> MAHHHHHHSAAISNLQEKQTDFGMRVFSQVAQNSKGSNLAFSPYGVATILAMAQLGAGGNTLKTLNAKLGFSLQERGMARQQRLLQRDISSEEGVELASGVMVERKMALEKGFRRGLGKAFQASPHQLDFSRPDQALDIINAWVSDHTAGTIPSFLSSGALTDETRMVLLNALHFQGLWKVPFDPKMTEERLFHCANGSSVPVPMMRLTHRFKYGEFVTPDGVDYDVIEVPYEGESLSMLLVSPFEPETPVSSLSSELTTQRLQQWRQEMRSVKRQLVLPRFTLDSEVELKSILIQMGLGDMFNLAKADFTRITTEQPLCVSKVLQKVKIEVNEEGTKASAATAAILFSRMAVEEITMNRPFLFLIHHKSTGAVLFMGQVN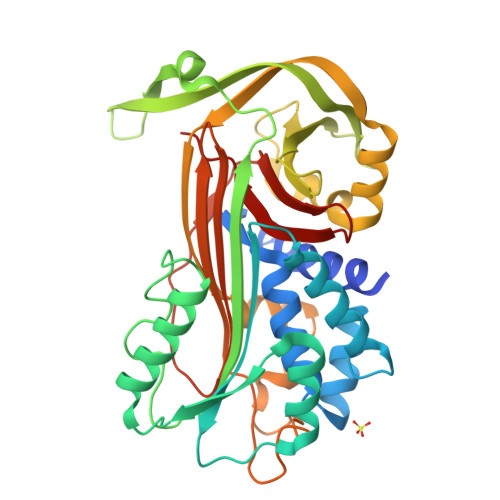QPQQH 3,5,6-trichloro-2-pyridinol | C5 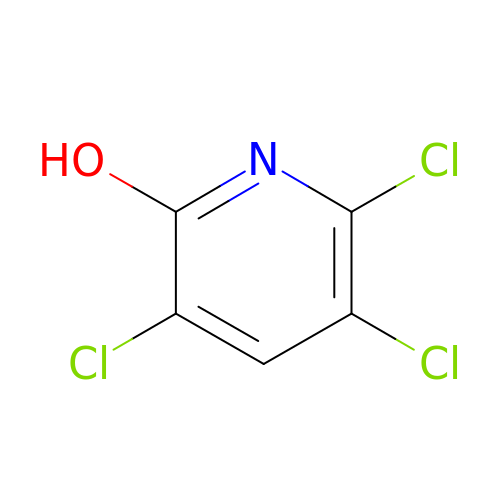H2 Cl3 N O | WCYYAQFQZQEUEN-UHFFFAOYSA-N> MHHHHH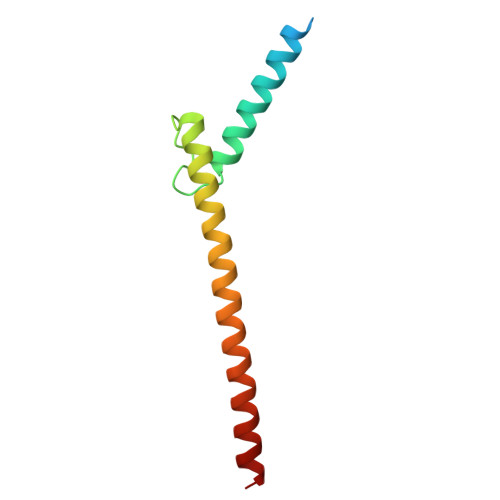HEENVKRRTHNVLERQRRNELKRSFFALRDQIPELENNEKAPKVVILKKATAYILSVQAEEQKLISEEDLLRKRREQLKHKLEQLRNS> MSDLVNKKFPAGDYKFQYIAISQSDADSESCKMPQTVEWSKLISENKKVIITGAPAAFSPTSTVSHIPGYINYLDELVKEKEVDQVIVVTVDNPFANQAWAKSLGVKDTTHIKFASDPGCAFTKSIGFELAVGDGVYWSGRWAMVVENGIVTYAAKETNPGTDVTVSSVESVLAHL;> MGHHHHHHMVTQLKSASEYDSALASGDKLVVVDFFATWCGPSKMIAPMIEKFAEQYSDAAFYKLDVDEVSDVAQKAEVSSMPTLIFYKGGKEVTRVVGANPA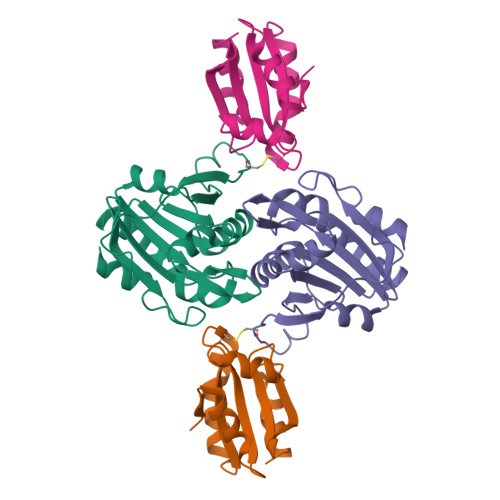AIKQAIASNV>GSHMMIQSQINRNIRLDLADAILLSKAKKDLSFAEIADGTGLAEAFVTAALLGQQALPADAARLVGAKLDLDEDSILLLQMIPLRGCIDDRIPTDPTMYRFYEMLQVYGTTLKALVHEKFGDGIISAINFKLDVKKV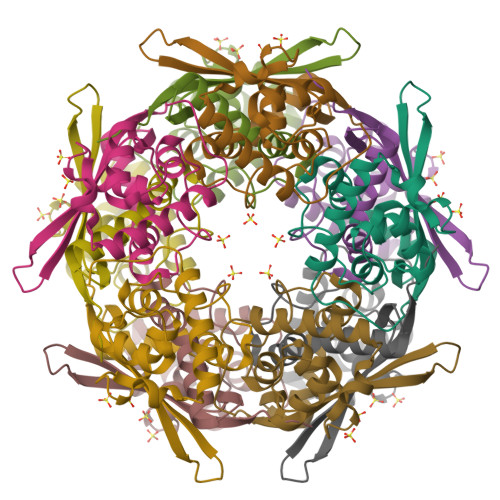ADPEGGERAVITLDGKYLPTKPF[10x]> MASPAPSWTRLDPQQERDVRELIRLVSGVQDEADPNFQLALHFAWSNFRFHRFLDVNSHKVEKTIEGIYEKFIIHSDLSKAASWKRLTDEFLNASLPSIKEIKTDAHYSILSLLLCLSDSPSNSNYVETPRNKEVEKKDDFDWGKYLMEGEEIDLGPNVDTPNWSEESEDEDDPQPLSREDSGIQVDRTPLEEQDQSRKPASRVSWKVDEPDARSWLEQHVVRQYWTTRSSKFPHSLHLHSNLAAVWDQHLYSSDPLYVPDDRVSVTETQVIRETLWLLSGVKKLFIFQLIDGKVAVRNNIMVTHLTHSCLRSVLEQIAAYGQVVFRLQEFIDEVMGHSSESTLPGNGSVPKKSTDAPFRTYQAFMWALYKYFISFKEELSEIEKCIINNDTTVTLAIVVDKLSPRLAQLKVLHKVFSTGVAEVPPDTRNVVRASHLLNTLYKAILEYDNVGEASEQTVSLLFSLWVETVRPYLQIVDEWIVHGHLCDGAREFIIQRNKNVPVNHRDFWYATYTLYSVSEKTENEEKMSDNASASSGSDQGPSSRQHTMVSFLKPVLKQIIMAGKSMQLLKNLQCAESTTCQAMARDAERKSLYTLFLESVQSRLRHGEDATAQALTEQQATRETLIKMQSIAERHLELDDVHDPLLAINFARLY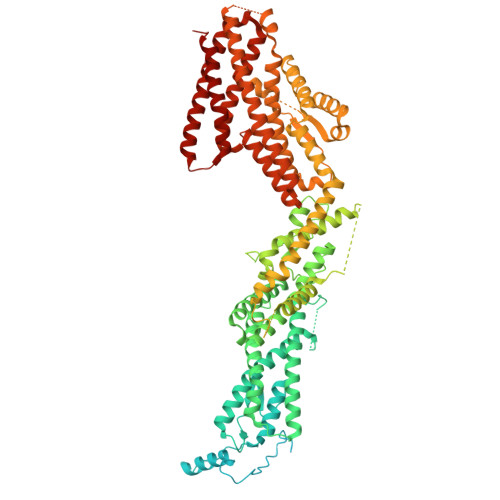LEQSDFHEKFAGGDICVDRSSESVTCQTFELTLRSCLYPHIDKQYLDCCGNLMRTLKKDYRLVEYLQAMRNFFLMEGGDTMYDFYTSIFDKIREKETWQNVSFLNVQLQEAVGQRYPEDSSRLSISFENTDTAKKKLPVHTLDGLTLSYKVPWPVDIVISLECQKIYNQVFLLLLQIKWAKYSLDVLLFGELASSAEKPQSKEGLLSGQDTAAQFGPQKEPVRQQIHRMFLLRVKLMHFVNSLHNYIMTRILHSTGLEFQHQVEEAKDLDQLIKIHYRYLSTIHDRCLLREKVSFVKEAIMKVLNLALMFADGWQAGLGAWHGISSAVTHGWHGTKLNIFSAVNTSDLIVIHFHHMQLRNRNLFWTVLKPLVYYLDKWILFPLGIIG>GSQIPASEQETLVRPKPLLLKLLKSVGAQKDTYTMKEVLFYLGQYIMTKRLYDEKQQHIVYCSNDLLGD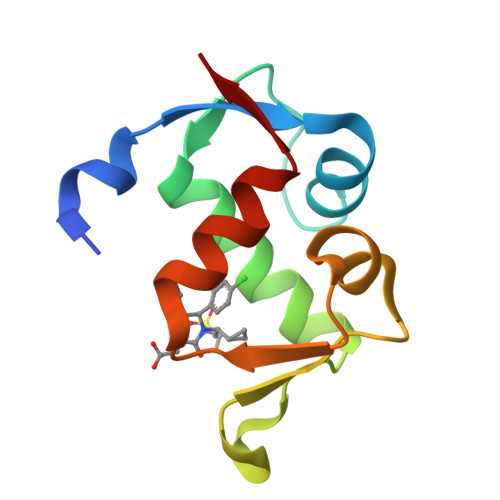LFGVPSFSVKEHRKIYTMIYRNLVVVN[6x]>MRSVEQQLSIVTEAAVAPEPVRIAIAEALGLMCAEEVQASRALPGFAQAAIDGYAVRAVDVGGEKSL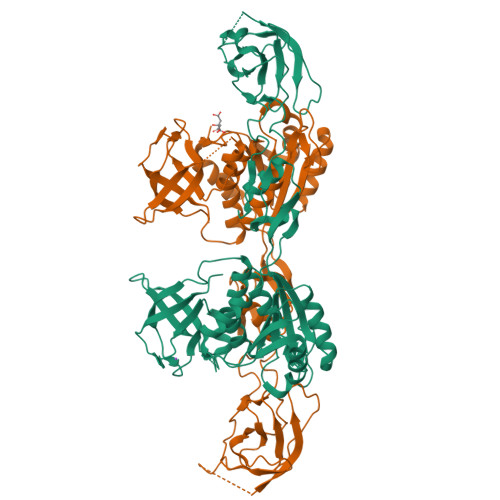SQQLPVAPPEKSLPVVGEVAAGSQQPLRLQPKQAVMVHTGAPLPMLADAVLPMAWSDRGRKRVTAQRPVRSGEFVRKEGDDIQPGDIAVSAGAVLGPAQIGLLAAVGRSKVLVYPRPRMSVISVGAELVDIDRQPGLGQVYDVNSYSLAAAGREAGADVYRYGIAAGEPRRIKEIIESQMLRSEIIVITGAVGGAGSAGVRQVLNELGDIDTERVAMHPGSVQGFGLLGENKIPCFLLPSNPVASLVIFETFVRPVVRMSLGKSNAARRVVRARALNHVVSVAGRKGFIRSRLMRDAETQDYLVEALGGATGAPSHLLAGLSEANGMIRIPEDVTEIRPGDVVDVIFLAQGR[2x]>[2x]GSIKTRIEEVQLQFLTGNTELTHLKVSNDQLIVTTQRTIYRINLQDPAIVNHFDCPLSKELETIMNVHVSPMGSVILIRTNFGRYMLLKDGEFTQLNKIKNLDLSSLHWINETTFLMGIKKTPKLYRVELTGKDITTKLWYENKKLSGGIDGIAYWEGSLLLTIKDNILYWRDVTNMKFPLVLPDESEQFERLKHHAIKKFDSYNGLFAWVTSNGIVFGDLKEKQ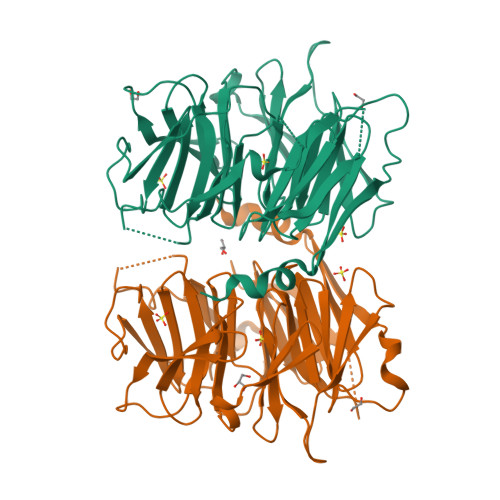MEKDPASNNFGKFLSSSKVLLNFELPDYQNDKDHLIKDIVLTAFHILLLRKNTVTMVSQLNNDVVFHETIPRHQLTGSNTDSNEKFLGLVRDSVKETFWCFSNINVFEIIIENEPNSVWNLLVR> DASIATFKGSEYFCYDLSQNPIQSSSDEITLSFKTLQRNGLMLHTGKSADYVNLALKNGAVSLVINLGSGAFEALVEPVNGKFNDN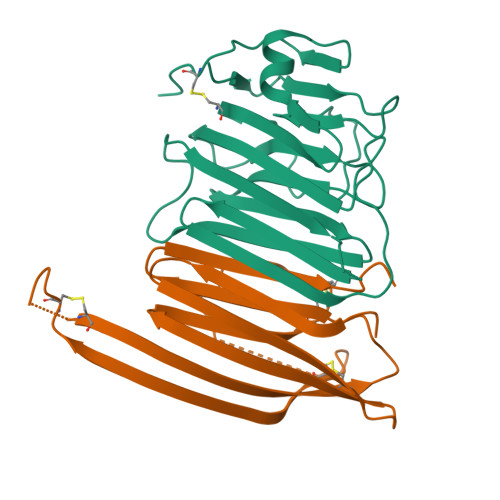AWHDVKVTRNLRQHSGIGHAMVTISVDGILTTTGYTQEDYTMLGSDDFFYVGGSPSTADLPGSPVSNNFMGCLKEVVYKNNDVRLELSRLAKQGDPKMKIHGVVAFKCAALEVLFQ;> DAAQPAARDFGWGDFHSNIKTVKLNLLITGKIVDHGDGTFSVYFRHDSTGQGDVSVSLVPPTKIVEFDLAQQTVIDAKDSKSFNCRIEYEKVDKATKNTLCNYDPSKTCYQEQTQSHVSWLCSKPFKVICIYISFYSTDYKLVQKVCPDYNYHSDTPYFPSGLEVLFQ> DWVIPPISCPENEKGEFPKNLVQIKSNRDKETKVFYSITGQGADKPPVGVFIIERETGWLKVTQPLDREAIAKYILYSHAVSSNGEAVEDPMEIVITVT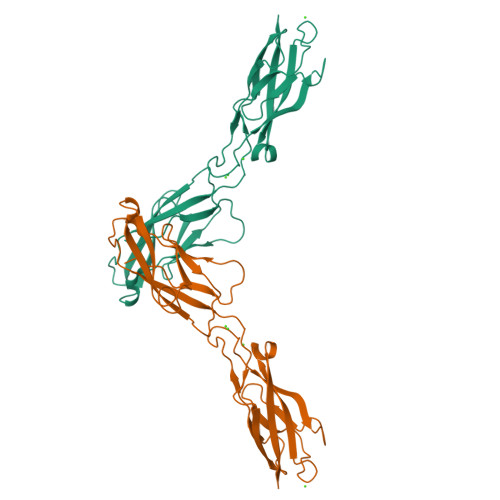DQNDNRPEFTQEVFEGSVAEGAVPGTSVMKVSATDADDDVNTYNAAIAYTIVSQDPELPHKNMFTVNRDTGVISVLTSGLDRESYPTYTLVVQAADLQGEGLSTTAKAVITVKD>[2x]IADVANDKPYTVAVSGKTITVESPAAGLTIFDMNGRRVAT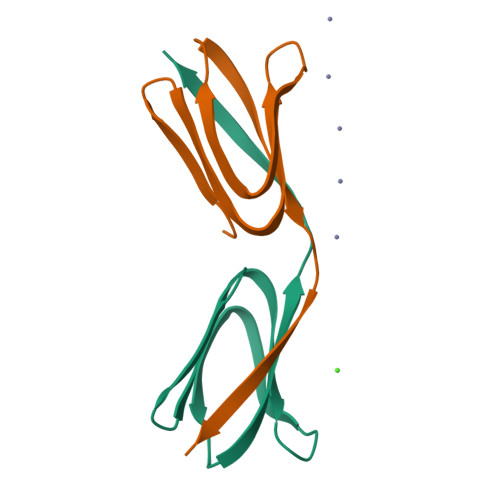AKNRMVFEAQNGVYAVRIATEGKTYTEKVIVK(2S)-2-hexyl-N-[(3S)-2-oxooxolan-3-yl]decanamide 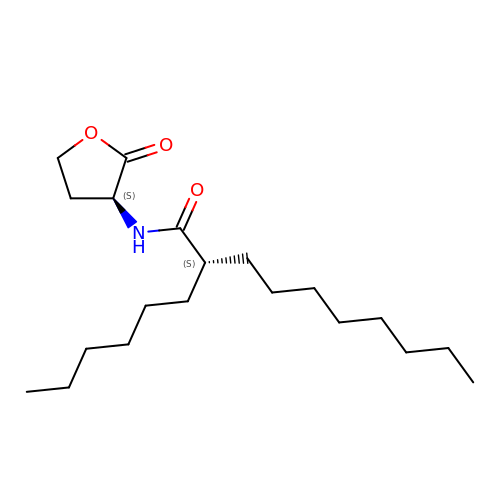| C20 H37 N O3 | XGYNUFAUHRHVSH-ROUUACIJSA-N>SDAIKMFVGQVPRTWSEKDLRELFEQYGAVYEINVLRDRSQNPPQSKGCCFVTFYTRKAALEAQNAL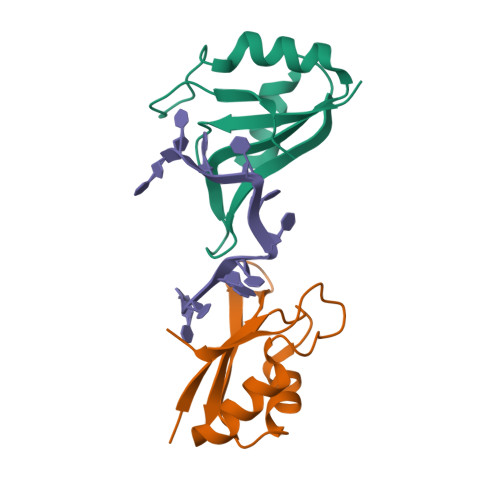HNMKVLPGMHHPIQMKPADSE[4x]>[4x]MINEIEIKRKFGRTLK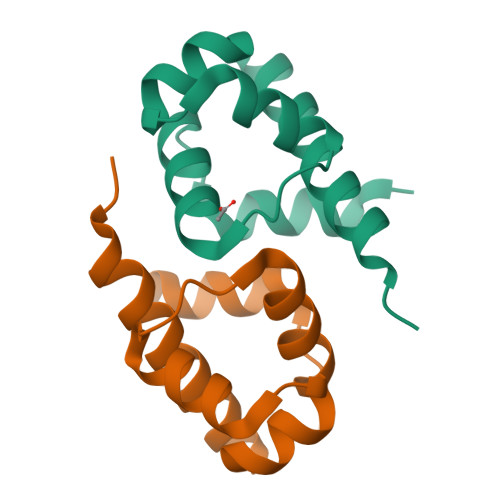KIRTQKGVSQEELADLAGLHRTYISEVERGDRNISLINIHKICAALDIPASTFFRKMEEEN> MRTDW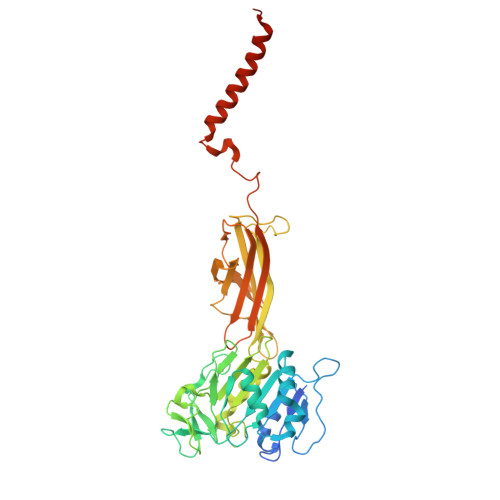NFFFCILLQAIFVVGTQTSRTLVLYDQSTEPLEEYSVYLKDLEQRNYKLEYLDINSTSTTVDLYDKEQRLFDNIIVFPTKGGKNLARQIPVKQLIKFFENEGNILCMSSPGAVPNTIRLFLNELGIYPSPKGHVIRDYFSPSSEELVVSSNHLLNKYVYNARKSEDFVFGESSAALLENREQIVPILNAPRTSFTESKGKCNSWTSGSQGFLVVGFQNLNNARLVWIGSSDFLKNKNQDSNQEFAKELLKWTFNEKSVIKSVHAVHSHADGTSYDEEPYKIKDKVIYSVGFSEWNGEEWLPHIADDIQFELRQVDPYYRLTLSPSGNDSETQYYTTGEFILPDRHGVFTFLTDYRKIGLSFTTDKDVKAIRHLANDEYPRSWEISNSWVYISAICGVIVAWIFFVVSFVTTSSVGKKLETFKKTN>MHHHHHHMTIALNNVVAVVTGAAGGIGRELVKAMKAANAIVIATDMAPSADVEGAD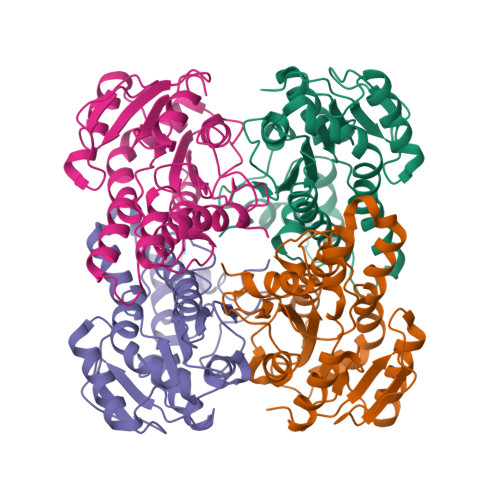HYLQHDVTSEAGWKAVAALAQEKYGRVDALVHNAGISIVTKFEDTPLSDFHRVNTVNVDSIIIGTQVLLPLLKEGGKARAGGASVVNFSSVAGLRGAAFNAAYCTSKAAVKMLSKCLGAEFAALGYNIRVNSVHPGGIDTPMLGSLMDKYVELGAAPSREVAQAAMEMRHPIGRMGRPAEMGGGVVYLCSDAASFVTCTEFVMDGGFSQV[16x]Gedatolisib | C32 H41 N9 O4 | 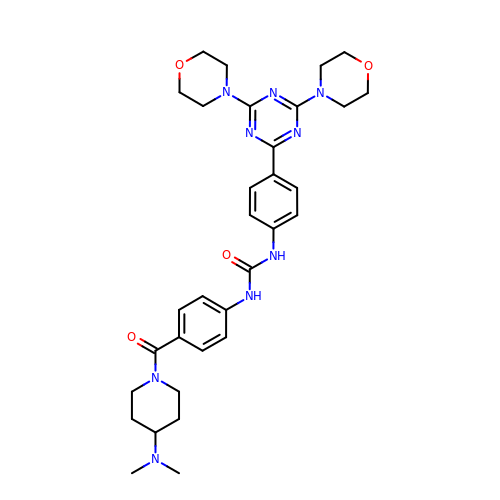DWZAEMINVBZMHQ-UHFFFAOYSA-N> SLLLDDVDNEMAAIAMQGFRSMIEQFNVNNPATAKELQAMEAQLTAMSDQLVGADGELPAEIQAIKDALAQALKQPSADGLA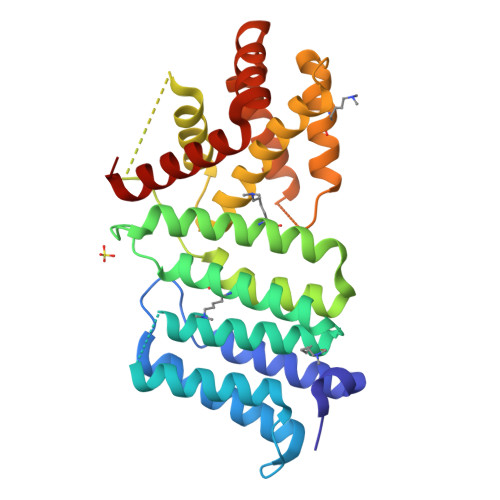TAMGQVAFAAAKVGGGSAGTAGTVQMNVKQLYKTAFSSTSSSSYAAALSDGYSAYKTLNSLYSESRSGVQSAISQTANPALSRSVSRSGIESQGRSADASQRAAETIVRDSQTLGDVYSRLQVLDSLMSTIVSNPQANQEEIMQKLTASISKAPQFGYPAVQNSVDSLQKFAAQLEREFVDGERSLAESQENAFRKQPAFIQQVLVNIASLFSGYLS> LKESPSGYLRSGEGDTGCGELVWVGEPLTLRTAETITGKYGVWMRDPKPTYPYTQETTWRIDTVGTDVRQVFEYDLISQFMQGYPSKVHILPRPLESTG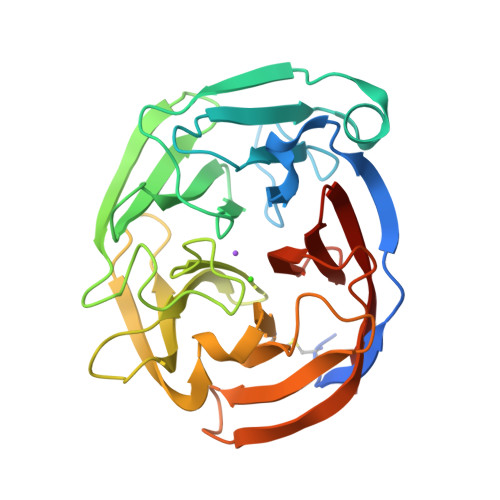AVVYSGSLYFQGAESRTVIRYELNTETVKAEKEIPGAGYHGQFPYSWGGYTDIDLAVDEAGLWVIYSTDEARGAIVLSKLNPENLELEQTWETNIRKQSVANAFIICGTLYTVSSYTSADATVNFAYDTGTGISKTLTIPFKNRYKYSSMIDYNPLEKKLFAWDNLNMVTYDIKLSKM>[6x]GPGKTDSSF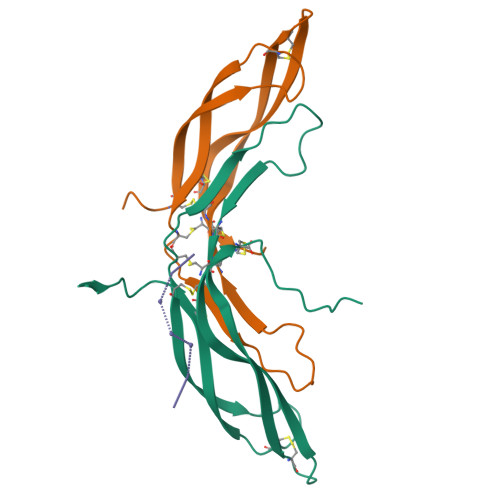IMDSDPRRCMRHHYVDSISHPLYKCSSKMVLLARCEGHCSQASRSEPLVSFSTVLKQPFRSSCHCCRPQTSKLKALRLRCSGGMRLTATYRYILSCHCEECNSGTETSQVAPA;> EEEEEEE;> EEEE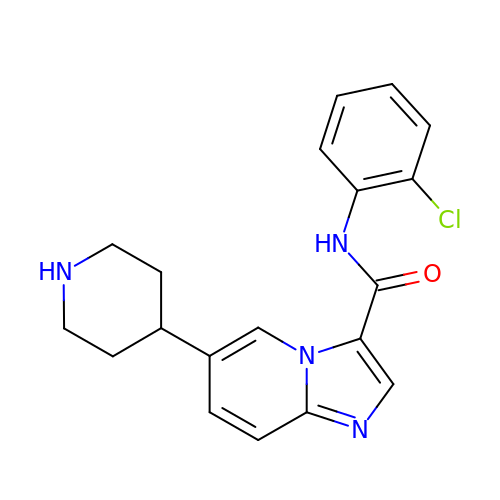~{N}-(2-chlorophenyl)-6-piperidin-4-yl-imidazo[1,2-a]pyridine-3-carboxamide | C19 H19 Cl N4 O | DGSMEFWSLXFLQA-UHFFFAOYSA-N> MKKISRKEYVSMYGPTTGDKVRLGDTDLIAEVEHDYTIYGEELKFGGGKTLREGMSQSNNPSKEELDLIITNALIVDYTGIYKADIGIKDGKIAGIGKGGNKDMQDGVKNNLSVGPATEALAGEGLIVTAGGIDTHIHFISPQQIPTAFASGVTTMIGGGTGPADGTNATTITPGRRNLKWMLRAAEEYSMNLGFLAKGNASNDASLADQIEAGAIGFKIHEDWGTTPSAINHALDVADKYDVQVAIHTDTLNEAGCVEDTMAAIAGRTMHTFHTEGAGGGHAPDIIKVAGEHNILPASTNPTIPFTVNTEAEHMDMLMVCHHLDKSIKEDVQFADSRIRPQTIAAED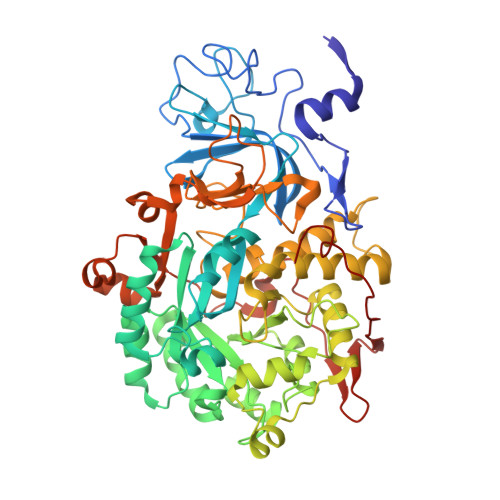TLHDMGIFSITSSDSQAMGRVGEVITRTWQTADKNKKEFGRLKEEKGDNDNFRIKRYLSKYTINPAIAHGISEYVGSVEVGKVADLVLWSPAFFGVKPNMIIKGGFIALSQMGDANASIPTPQPVYYREMFAHHGKAKYDANITFVSQAAYDKGIKEELGLERQVLPVKNCRNITKKDMQFNDTTAHIEVNPETYHVFVDGKEVTSKPANKVSLAQLFSIF>MTVGAVVVDHEGNVAAAVSSGGLALKHPGRVGQAALYGCGCWAENTGAHNPYSTAVSTSGCGEHLVRTILARECSHALQAEDAHQALLETMQNKFISSPFLASEDGVLGGVIVLRSCRCS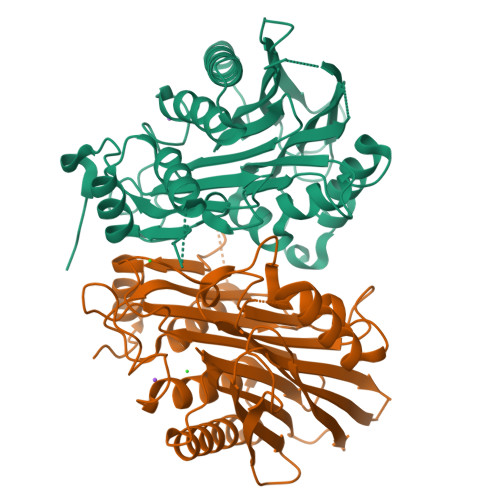AEPDSSQNKQTLLVEFLWSHTTESMCVGYMSAQDGKAKTHISRLPPGAVAGQSVAIEGGVCRLEGSGSGGFVLVHAGAGYHSESKAKEYKHVCKRACQKAIEKLQAGALATDAVTAALVELEDSPFTNAGMGSNLNLLGEIECDASIMDGKSLNFGAVGALSGIKNPVSVANRLLCEGQKGKLSAGRIPPCFLVGEGAYRWAVDHGIPSCPLEHHHHHH[2x]> 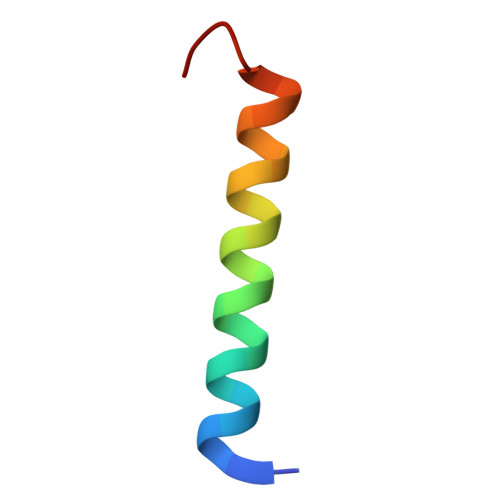MSAGVITGVLLVFLLLGYLVYALINAEAF> MPLLSASIVSAPVVTSETYVDIPGLYLDVAKAGIRDGKLQVILNVPTPYATGNNFPGIYFAIATNQGVVADGCFTYSSKVPESTGRMPFTLVATIDVGSGVTFVKGQWKSVRGSAMHIDSYASLSAIWGTA

The bacterial lectin BC2L‐C expressed in B. cenocepacia is an interesting drug target involved in bacterial adhesion and subsequent deadly infection to the host. For BC2L‐C, the C‐terminal domain (LecB like) specifically binds to mannose, while the N‐terminal domain (BC2L‐C‐nt) has been structurally characterized as a novel fucose‐binding domain with a trimeric TNF‐α‐like architecture. Thus, BC2L‐C represents a novel type of superlectin with dual specificity for fucose and mannose in the N‐ and C‐terminal domains, respectively. BC2L‐C as a virulence factor binds to carbohydrates present on the epithelial cells of the host.

The crystal structures of complexes evidenced some promising pockets on the protein surface near the fucose binding site. The occurrence of such pockets in the apo‐protein needed to be verified and therefore, we solved the crystal structure of the apo form of BC2L‐C‐nt at high resolution (1.5 Å). The asymmetric unit in the P63 space group contains one monomer and crystal symmetry was applied to build the trimer for comparison with other structures. Root‐mean‐squares values of 0.21 Å and 0.24 Å were obtained when comparing with the trimer complexed with MeSe‐α‐L‐Fuc and Globo‐H, respectively. Comparison of binding sites did not display significant differences in the amino acid of fucose binding pockets and environment. Only a minor difference is observed at the surface loop (Asn52‐Phe54), that is involved in the interaction with methyl group of N‐acetylgalactosamine (GalNAc) in the complex with Globo‐H. Likewise, small differences in the conformation of the N‐ and C‐terminal residues were noticed due to H‐bond interaction between them. The changes in the conformation of the termini further caused a small displacement (0.6 to 1.0 Å) of surface loops (Val28‐Asp35, Asp95‐Val100). Analysis of water molecules involved in bridging fucose to protein indicated that the more buried one (W1) is conserved in all structures, while the more exposed one (W2) moves by 1.9 Å in the apo structure. The new crystal structure therefore confirms that the region surrounding the fucose binding site is of interest for drug design.> SGRS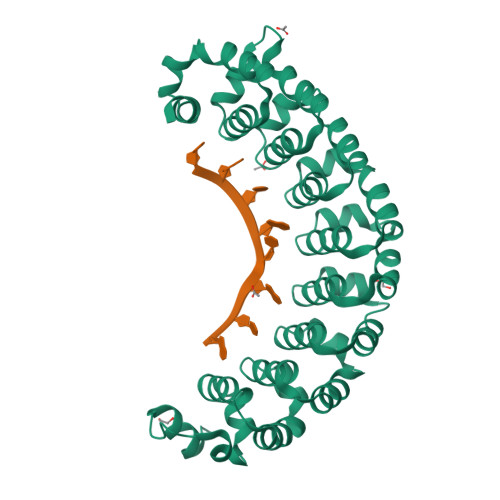RLLEDFRNQRYPNLQLRDLANHIVEFSQDQHGSRFIQQKLERATAAEKQMVFSEILAAAYSLMTDVFGNYVIQKFFEFGTPEQKNTLGMQVKGHVLQLALQMYGCRVIQKALESISPEQQQEIVHELDGHVLKCVKDQNGNHVVQKCIECVDPVALQFIINAFKGQVYSLSTHPYGCRVIQRILEHCTAEQTTPILDELHEHTEQLIQDQYGNYVIQHVLEHGKQEDKSILINSVRGKVLVLSQHKFASNVVEKCVTHATRGERTGLIDEVCTFNDNALHVMMKDQYANYVVQKMIDVSEPTQLKKLMTKIRPHMAALRKYTYGKHINAKLEK> MNNPAIQRIEDHIVKSPEDKREYRGLELANGIKVLLISDPTTDKSSAALDVHIGSLSDPPNIPGLSHFCEHMLFLGTKKYPKENEYSQFLSEHAGSSNAFTSGEHTNYYFDVSHEHLEGALDRFAQFFLCPLFDASCKDREVNAVDSEHEKNVMNDAWRLFQLEKATGNPKHPFSKFGTGNKYTLETRPNQEGIDVREELLKFHSTYYSSNLMAICVLGRESLDDLTNLVVKLFSEVENKNVPLPEFPEHPFQEEHLKQLYKIVPIKDIRNLYVTFPIPDLQQYYKSNPGHYLGHLIGHEGPGSLLSELKSKGWVNTLVGGQKEGARGFMFFIINVDLTEEGLLHVEDIILHMFQYIQKLRAEGPQEWVFQECKDLNAVAFRFKDKERPRGYTSKIAGKLHYYPLNGVLTAEYLLEEFRPDLIDMVLDKLRPENVRVAIVSKSFEGKTDRTEQWYGTQYKQEAIPEDVIQKWQNADLNGKFKLPTKNEFIPTNFEILALEKDATPYPALIKDTAMSKLWFKQDDKFFLPKACLNFEFFSPFAYVDPLHCNMAYLYLELLKDSLNEYAYAAELAGLSYDLQNTIYGMYLSVKGYNDKQPILLKKITEKMATFEIDKKRFEIIKEAYMRSLNNFRAEQPHQHAMYYLRLLMTEVAWTKDELKEALDDVTLPRLKAFIPQLLSRLHIEALLHGNITKQAALGVMQMVEDTLIEHAHTKPLLPSQLVRYREVQLPDRGWFVYQRRNEVHNNCGIEIYYQTDMQSTSENMFLELFCQIISEPCFNTLRTKEQLGYIVFSGPRRANGIQGLRFIIQSEKPPHYLESRVEAFLITMEKAIEDMTEEAFQKHIQALAIRRLDKPKKLSAECAKYWGEIISQQYNYDRDNIEVAYLKTLSKDDIIKFYKEMLAVDAPRRHKVSVHVLAREMDSCPVVGEFPSQNDINLSEAPPLPQPEVIHNMTEFKRGLPLFPLVKPHINFMAAKL

Insulysin (EC 3.4.24.56; also referred to as insulin-degrading enzyme or IDE) is a zinc metallopeptidase in the M16 family that has been extensively studied because of its role in cellular insulin degradation and amyloid beta peptide catabolism. IDE exists predominantly as a dimer in equilibrium with tetramers and to a lesser extent monomers. It is unique among the enzymes comprising the zinc metallopeptidase M16 family in that it exhibits allosteric kinetic behavior with substrate peptides increasing its activity. Crystal structures of human IDE (hIDE) complexed with peptides show that the enzyme consists of four structurally related domains that adopt a clamshell-like structure enclosing a large central chamber.

We report here the crystal structures of rat IDE (rIDE) and a catalytically compromised mutant form, rIDE-E111F. The structures of wild type and E111F rIDE are very similar to the published structures of peptide bound and unliganded human IDE (hIDE). The four structurally similar domains each have an α+β fold and arrange to form the same closed clamshell conformation as hIDE, with the N- and C-terminal halves of the clamshell connected by a single polypeptide chain. In the closed conformation, the two halves of the clamshell are in contact with one another forming an enclosed cavity, and the active site of the enzyme is accessible from this internal substrate-binding chamber. Bound peptides are presumably not seen associated with wild type rIDE because the polyhistidine fusion sequences are degraded by the active enzyme. Comparison of the ligand free rIDE structure and the rIDE-E111F structure with ligand bound at the distal and active sites suggests a likely structural basis for allosterism. As already noted, the crystallographic thermal factors for the first two domains of the ligand bound mutant are consistently higher than those for the unliganded enzyme. This difference may reflect a higher relative mobility of the two halves of the peptide bound enzyme, which would be consistent with a weakening of the interface. The observed conformational shift at the dimer interface between ligand free wild type enzyme and ligand bound rIDE-E111F reported here suggests a possible structural basis for this communication.5-(2-NITROPHENYL)-2-FUROIC ACID 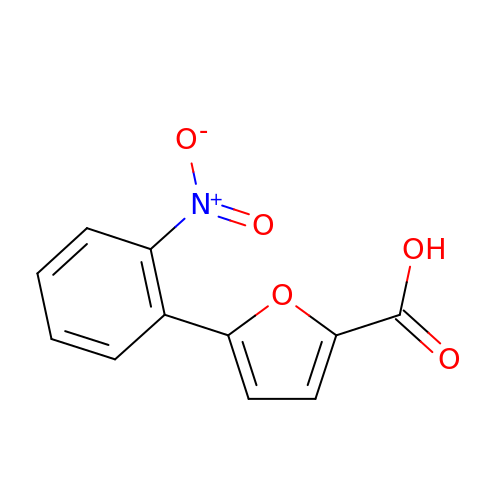| C11 H7 N O5 | XUFDYUSOQQYQRL-UHFFFAOYSA-N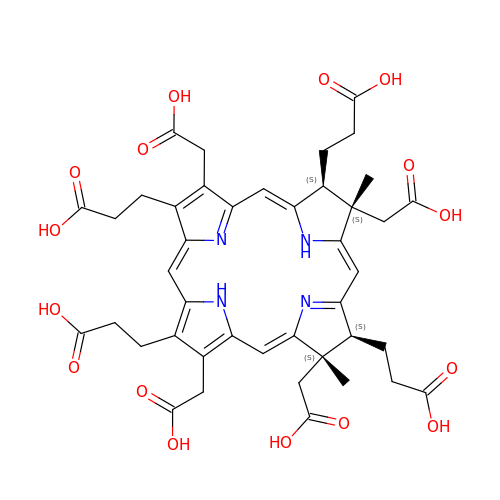3,3',3'',3'''-[(7S,8S,12S,13S)-3,8,13,17-tetrakis(carboxymethyl)-8,13-dimethyl-7,8,12,13-tetrahydroporphyrin-2,7,12,18-tetrayl]tetrapropanoic acid | C42 H46 N4 O16 | KWIZRXMMFRBUML-OWSSXZAMSA-N>CCGATAUCG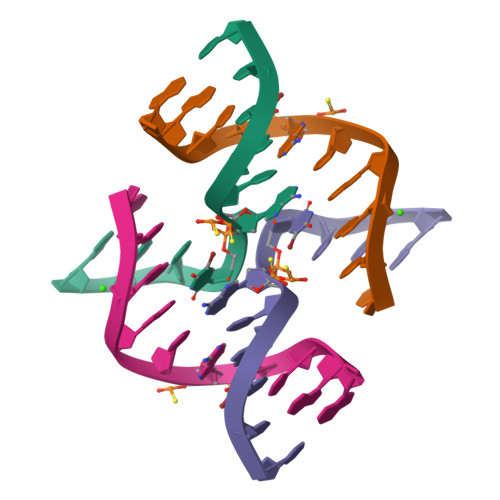G[2x]>MSHVPPHVPFELSGAELRDAIVQYATNPIYHDNLDWLNHDNPYRRQLRPQVLPHLDYDKVPGRENILNYASLAVQRLLTSVYEADLVFFPKSGLKGKEEDFRAFYSPANRALGERIRPALERYAFGFLDDEVETSGTWTAQSLDAYLDSLDTAGGAEQSPVEKAILGSADRERAARMWLVQFAPDFLSEASPMMRNVLGYYGPAQSEWFKVVIDEYGYGVHDTKHSTLFERTLESVGLESDLHRYWQYYLNSSLLLNNYFHYLGKNHELFFRYVGALYYTESSLVDFCRRADHLLREVFGDTVDTTYFTE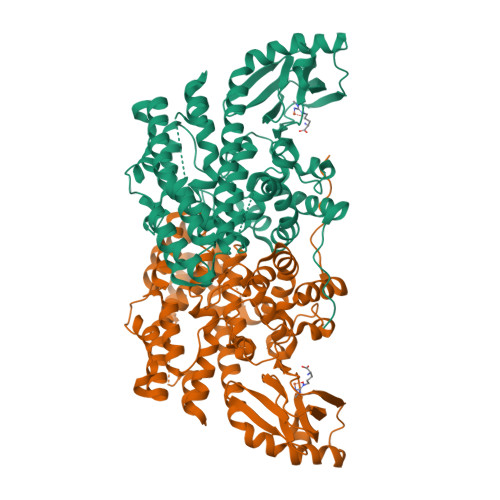HIHIDQHHGRMAREKIIKPLVEAHGDGIIPEIVRGIEEYRVLLEIGDFDFSEQIAWMDAQPELKKLHDPVFEGLKQGKVDAPVAHLVEPRGELSNTHCHDGDELCHIVSGTMRFESGLGSSLTLQAGEGVVIKRNRLHGANIESDECVYEIHSVGDYRKCL[2x]>GPLGSPEFMALAVAPWGRQWEEARALGRAVRMLQRLEEQCVDPRLSVSPPSLRDLLPRTAQLLREVAHSRRAAGGGGPGGPGGSGDFLLIYLANLEAKSRQVAALLPPRGRRSANDELFRAGSRLRRQLAKLAIIFSHMHAELH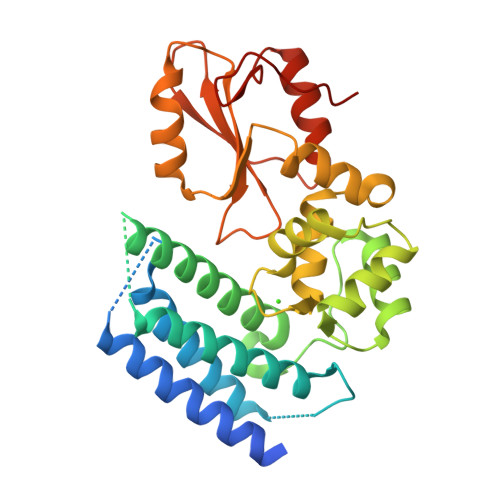ALFPGGKYCGHMYQLTKAPAHTFWRESCGARCVLPWAEFESLLGTCHPVEPGCTALALRTTIDLTCSGHVSIFEFDVFTRLFQPWPTLLKNWQLLAVNHPGYMAFLTYDEVQERLQACRDKPGSYIFRLSCTRLGQWAIGYVSSDGSILQTIPANKPLSQVLLEGQKDGFYLYPDGKTHNPDLTELG[2x]> MSE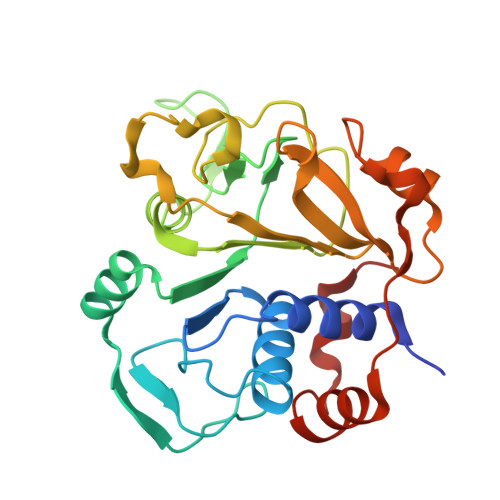TITEVTRAEYCAIACADIFSGAGEIMASPMATLPLIGARLARLTTEPDLLITDGEALIFADTPAVGAKAPIEGWMPFRKVFDVVASGRRHVVMGANQIDRHGNQNLSAFGPLQQPTRQMFGVRGAPGNTINHPTSYWVGKHTSRVFCDTVDIVSGVGYDQIDPENPAYRFHHLHRVVSNLGVFDFGGPDHTFRALSLHPGVTADQVADNTSFEVAGLADAGVTREPTDEELRLIREVLDPRSLRDREVSV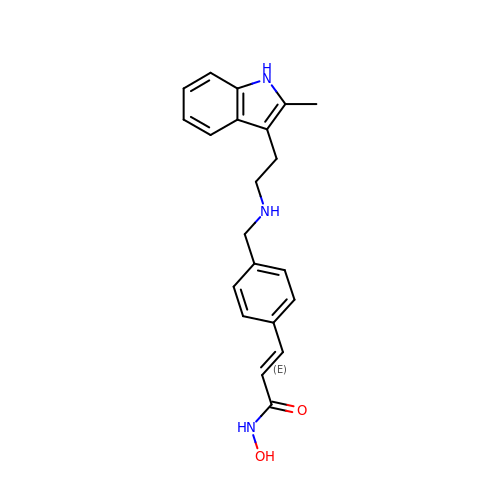Panobinostat | C21 H23 N3 O2 | FPOHNWQLNRZRFC-ZHACJKMWSA-N benzyl 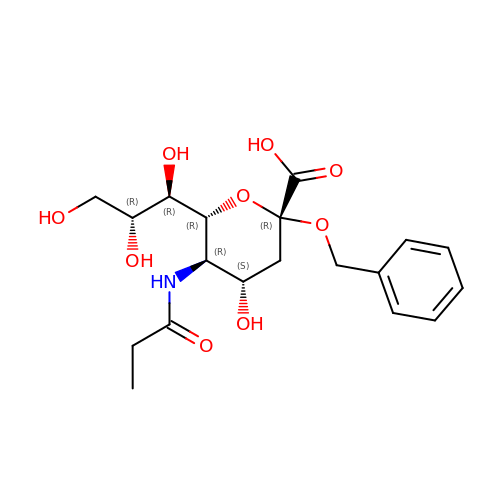3,5-dideoxy-5-(propanoylamino)-D-glycero-alpha-D-galacto-non-2-ulopyranosidonic acid | C19 H27 N O9 | XDURJXFZCXMSHL-YZKZVDITSA-N> MAHHHHHHMGGPPTIEELKREKIIPHVFPDENVDLTVDMYISFKSGKEVNHGNILDLAGTGSVPRNIKFSEEPPEDYCYILFMIDPDFPSRRRPDGRDYVHWAVSGIKSKELVKGTDKNCITLLPYVGPSIKKGTGLHRISFILSLVKEENKGNVTGVPLYRGEHYITRVKFNNCQSAYNVIQMNDMKIVGFNWCQMRR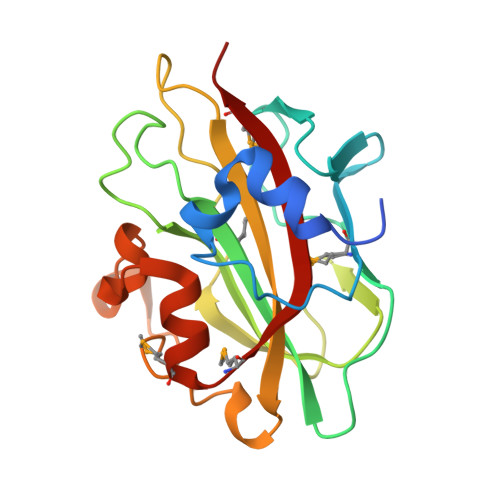K> XPPGPPGPRGPPGPPG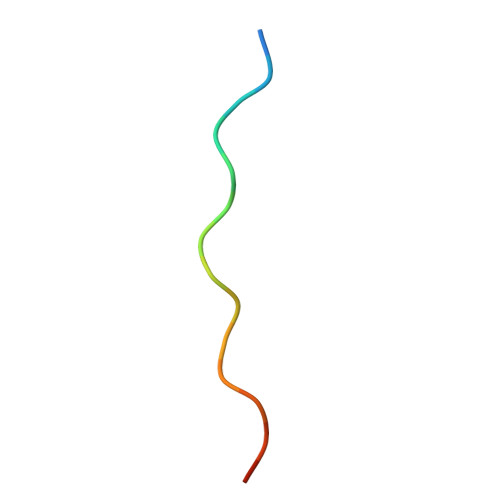X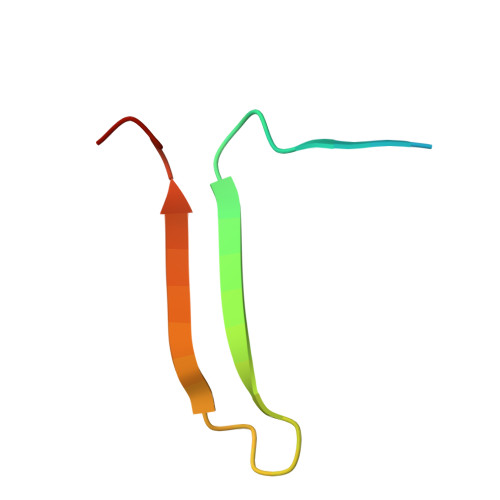> GPLVETRTIVRFNRPFLMIIVDNFTWSIFFMSKVTNPKQA>SDSGDGQDLRAFVHDSPEETETTQRLTKLLTNSPIPTEELVNNLPLFLRRHQMTDLLSMDALYRQVLDVPGVIMEFGVRFGRHLGTFAALRGVYEPYNPLRRIVGFDTFTGFPDVNDVDRVGPTAYQGRFAVPGGYPAYLKEVLDAHECSDFFGHVTQRSVLVEGDVRETVPRYLAENPQTVIALAYFDLDLYEPTKAVLEAIRPYLTKGSIVAFDELDNPKWPGENIAMRKVLGLDHAPLRLLPGRPAPAYLRW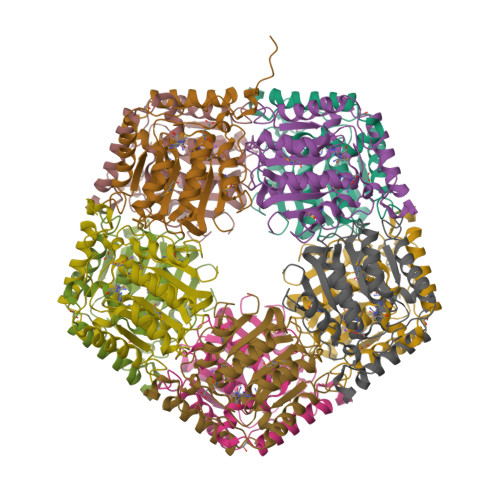GD[10x]> SMATKIDKEACRAAYNLVRDDGSAVIWVTFKYDGSTIVPGEQGAEYQHFIQQCTDDVRLFAFVRFTTGDAMSKRSKFALITWIGENVSGLQRAKTGTDKTLVKEVVQNFAKEFVISDRKELEEDFIKSELKKAGGANYDAQ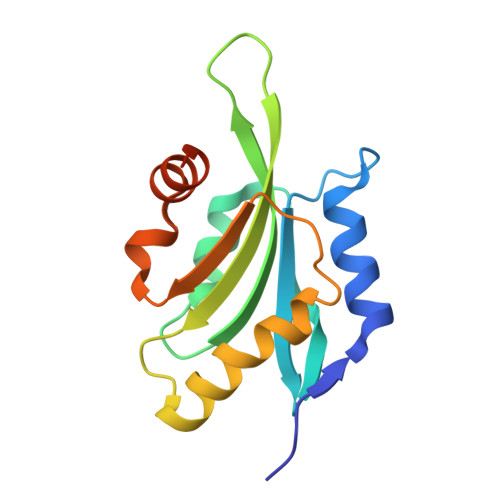TE> SLQPLPPTAFTPNGTYLQHLARDPTSGTLYLGATNFLFQLSPGLQLEATVSTGPVLDSRDCLPPVMPDECPQAQPTNNPNQLLLVSPGALVVCGSVHQGVCEQRRLGQLEQLLLRPERPGDTQYVAANDPAVSTVGLVAQGLAGEPLLFVGRGYTSRGVGGGIPPITTRALWPPDPQAAFSYEETAKLAVGRLSEYSHHFVSAFARGASAYFLFLRRDLQAQSRAFRAYVSRVCLRDQHYYSYVELPLACEGGRYGLIQAAAVATSREVAHGEVLFAAFSSAAPPTVGRPPSAAAGASGASALCAFPLDEVDRLANRTRDACYTREGRAEDGTEVAYIEYDVNSDCAQLPVDTLDAYPCGSDHTPSPMASRVPLEATPILEWPGIQLTAVAVTMEDGH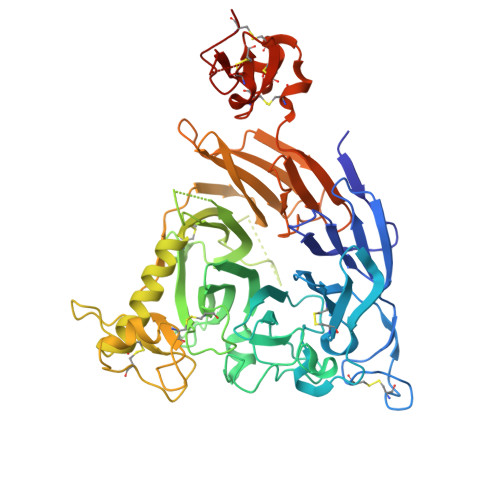TIAFLGDSQGQLHRVYLGPGSDGHPYSTQSIQQGSAVSRDLTFDGTFEHLYVMTQSTLLKVPVASCAQHLDCASCLAHRDPYCGWCVLLGRCSRRSECSRGQGPEQWLWSFQPELGCLQTRENLYFQ>GSTGSMVKSGKARAHTNIALIKYWGKADETYIIPMNNSLSVTLDRFYTETKVTFDPDFTEDCLILNGNEVNAKEKEKIQNYMNIVRDLAGNRLHARIESENYVPTAAGLASSASAYAALAAACNEALSLNLSDTDLSRLARRGSGSASRSIFGGFAEWEKGHDDLTSYAHGINSNGWEKDLSMIF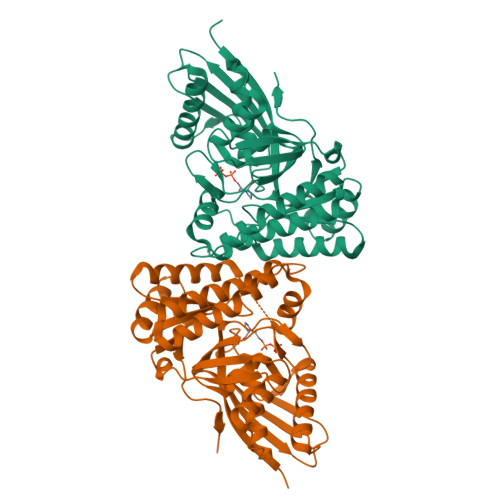VVINNQSKKVSSRSGMSLTRDTSRFYQYWLDHVDEDLNEAKEAVKNQDFQRLGEVIEANGLRMHATNLGAQPPFTYLVQESYDAMAIVEQCRKANLPCYFTMDAGPNVKVLVEKKNKQAVMEQFLKVFDESKIIASDIISSGVEIIK[2x]>[4x]PNYKLTYFNMRGRAEIIRYIFAYLDIQYEDHRIEQADWPEIKSTL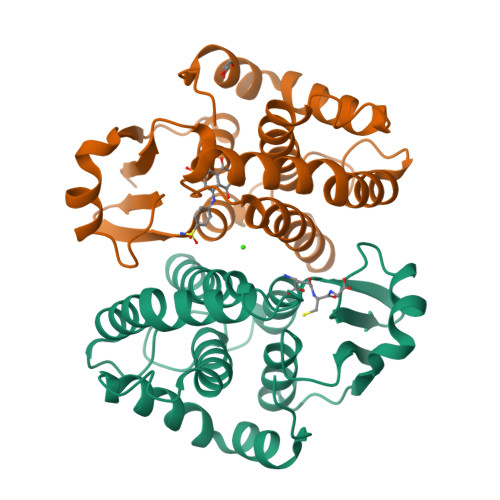PFGKIPILEVDGLTLHQSLAIARYLTKNTDLAGNTEMEQCHVDAIVDTLDDFMSCFPWAEKKQDVKEQMFNELLTYNAPHLMQDLDTYLGGREWLIGMSVTWADFYWEICSTTLLVFKPDLLDNHPRLVTLRKKVQAIPAVANWIKRRPQTKL1-(3-deoxy-3-fluoro-beta-D-glucopyranosyl)-4-[(phenylcarbonyl)amino]pyrimidin-2(1H)-one | C17 H18 F N3 O6 | 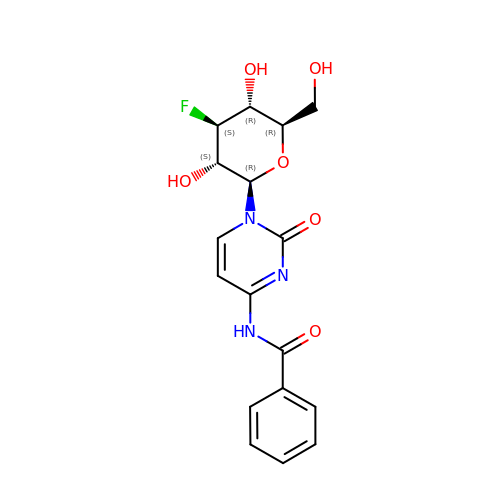PUCZITRLESUWFB-PBEGBBSFSA-N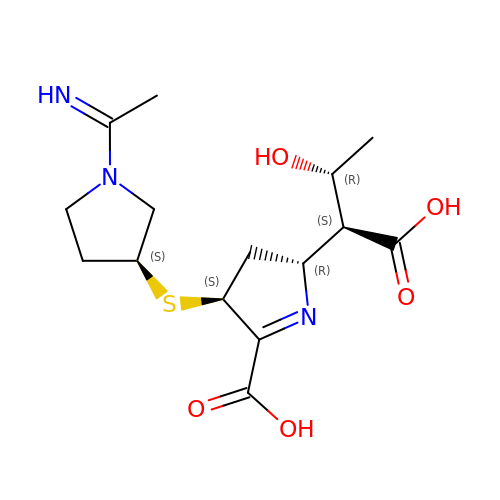(2R,4S)-2-[(2S,3R)-1,3-bis(oxidanyl)-1-oxidanylidene-butan-2-yl]-4-[(3S)-1-ethanimidoylpyrrolidin-3-yl]sulfanyl-3,4-dihydro-2H-pyrrole-5-carboxylic acid | C15 H23 N3 O5 S | ZWNVBHGNWGLVDB-DXBWQDCPSA-N> GSKVEDPKDFPSELLSFLSHAVFSNRTLACFAIYTTKEKAALLYKKIMEKYSVTFISRHNSYNHNILFFLTPHRHRVSAINNYAQKLCTFSFLICKGVNKEYLMYSALTRDPFS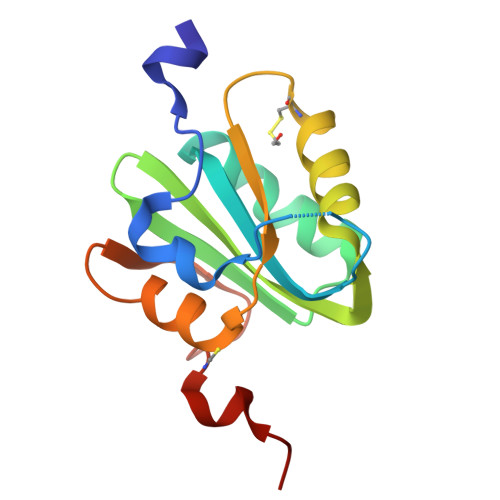VIEESLPGGLKEHDFNPESS> MDELYRQSLEIISRYLREQATGAKDTKPMGRSGATSRKALETLRRVGDGVQRNHETAFQGMLRKLDIKNEDDVKSLSRVMIHVFSDGVT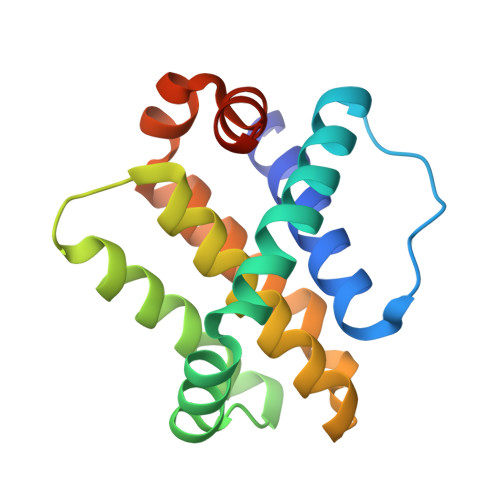NWGRIVTLISFGAFVAKHLKTINQESCIEPLAESITDVLVRTKRDWLVKQRGWDGFVEFFHVSRGKL> MRRHYRDLIRNTPMPDTPQDIADLRALLDEDEAEMSVVFSDPSQPDNPMIYVSDAFLVQTGYTLEEVLGRNCRFLQGPDTNPHAVEAIRQGLKAETRFTIDILNYRKDGSAFVNRLRIRPIYDPEGNLMFFAGAQNPVLEHHHHHH

Light, oxygen, voltage (LOV) domains are widely distributed in plants, algae, fungi, bacteria, and represent the photo-responsive domains of various blue-light photoreceptor proteins. Blue-light absorption triggers the formation of a transient adduct between the FMN-C4a atom and the sulfur atom of a strictly conserved cysteine residue in the LOV domain active site. Here, we report on the identification of an unusual short LOV protein DsLOV from the marine phototrophic α-proteobacterium Dinoroseobacter shibae DFL12T. Our data suggest that photopigment synthesis in D. shibae is primarily controlled by blue-light with the short LOV photoreceptor DsLOV acting as a key regulator.

Monoclinic crystals of the DsLOV protein were obtained in the dark, which diffracted to a resolution of 1.5 Å. In addition, a noncanonical structural element designated as the N-cap is present that includes a N-terminal turn (residues 20–23), helix (A´α, residues 24–27) and a connecting loop (28–35). The most probable higher-order assembly proposed by PISA analysis is a dimer, where the N-terminal A´α helix is part of the dimer interface that is unique amongst LOV protein structures. The buried surface area of ~950 Å2 involves a set of interchain interactions between charged residues (D20-OD2…NH1-R119´, 3.4 Å) (residues in italics with prime refer to those from the symmetry equivalent molecule), hydrogen bonds (D20-O…N-Y122´, 2.7 Å, A22-N…O-Y122´, 2.8 Å) and several hydrophobic interactions between residues in the N-terminal cap (including helix A´α) and the β-scaffold of the opposite subunit (Hβ and Iβ). Surprisingly, the chromophore bound in the DsLOV structure is RBF and not FMN; where both are identical except for the terminal phosphate group that is absent in RBF. We suspect that the FMN bound to the DsLOV protein in solution got hydrolyzed to RBF during the crystallization time period of several weeks in acidic conditions. Mainly, residues in the 310 Eα-helix (N71, R73, Q76), Hβ-strand (N104, N114), and Iβ strand (Q135) constitute most of the hydrogen bonding interactions with the RBF molecule. The double occupancy of M49 is indicative of structural flexibility of the respective residue in the dark.> MQAAALLLLVLRAITSIEAAADDVNPDDNKEDFAVLCALAALANLQTTVPSIDTSGLAAYDNLQQLNLSLSSKEWKSLFNKAADSNGSPKQPPEGFQSDPTWRKQWPIWVTAAAALKAENKEAAVLARAGLTNAPEELRNRARLALIPLLAQAEQIRDRLSEIQKQNEDTTPTAIAKALNKAVYGQDKETGAVYNSADCFSGNVADSTQNSCKAGNQASKATTVAATIVCVCHKKNGGNDAANACGRLINHQSDAGANLATASSDFGDIIATCAARPPKPLTAAYLDSALAAVSARIRFKNGNGYLGKFKATGCTGAAAEGLCVEYTALTAATMQNFYKIPWVKEISNVAEALKRTEKDAAESTLLSTWLKASENQGNSVAQK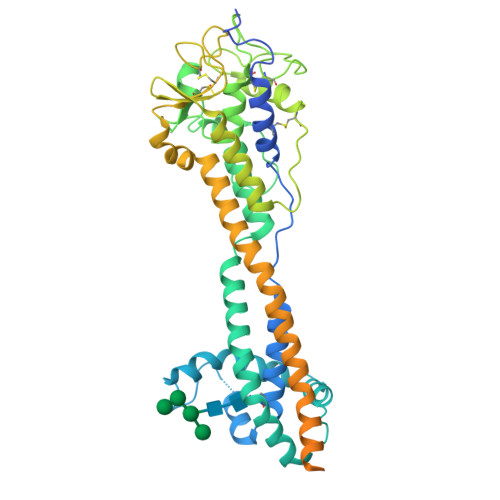LIKVGDSKAVPPAQRQTQNKPGSNCNKNLKKSECKDSDGCKWNRTEETEGDFCKPKETGTENPAAGTGEGAAGANTETKKCSDKKTEGDCKDGCKWDGKECKDSSILATKKFALTVVSAAFVALLF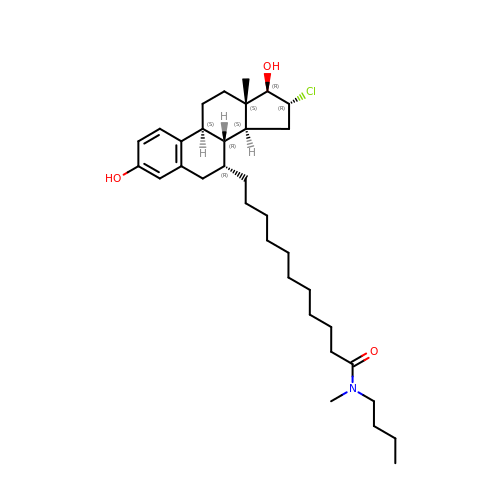N-butyl-11-[(7alpha,9beta,13alpha,14beta,16alpha,17alpha)-16-chloro-3,17-dihydroxyestra-1,3,5(10)-trien-7-yl]-N-methylundecanamide | C34 H54 Cl N O3 | FQJIZXBCOKNLMR-FTAPQOLWSA-N> MLNPKVAYMVWMTCLGLTLPSQAQSNDYRPSYHFTPDQYWMNEPNGLIKIGSTWHLFFQHNPTANVWGNICWGHATSTDLMHWAHKPTAIADENGVEAFTGTAYYDPNNTSGLGDSANPPYLAWFTGYTTSSQTQDQRLAFSVDNGATWTKFQGNPIISTSQEAPHDITGGLESRDPKVFFHRQSGNWIMVLAHGGQDKLSFWTSADTINWTWQSDLKSTSINGLSSDITGWEVPDMFELPVEGTEETTWVVMMTPAEGSPAGGNGVLAITGSFDGKSFTADPVDASTMWLDNGRDFDGALSWVNVPASDGRRIIAAVMNSYGSNPPTT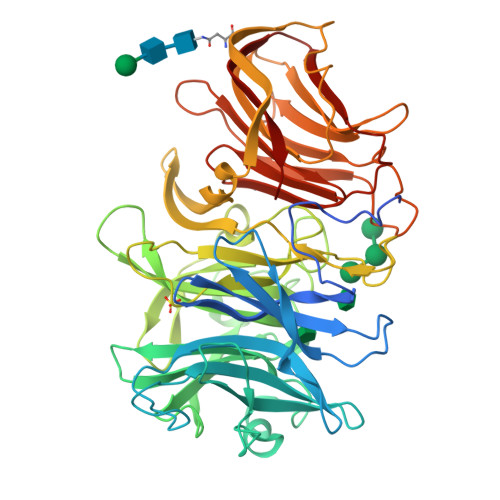TWKGMLSFPRTLSLKKVGTQQHFVQQPITELDTISTSLQILANQTITPGQTLLSSIRGTALDVRVAFYPDAGSVLSLAVRKGASEQTVIKYTQSDATLSVDRTESGDISYDPAAGGVHTAKLEEDGTGLVSIRVLVDTCSVEVFGGQGEAVISDLIFPSDSSDGLALEVTGGNAVLQSVDVRSVSLE>[2x]SNAMRKTKTEALKTKEHLMLAALETFYRKGIARTSLNEIAQAAGVTR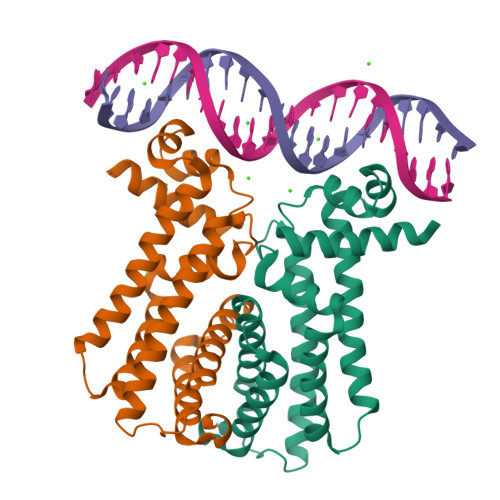GALYWHFKNKEDLFDALFQRICDDIENCIAQDAADAEGGSWTVFRHTLLHFFERLQSNDIHYKFHNILFLKCEHTEQNAAVIAIARKHQAIWREKITAVLTEAVENQDLADDLDKETAVIFIKSTLDGLIWRWFSSGESFDLGKTAPRIIGIMMDNLENHPCLRRK> SSETWRFDDGASLSYDWAAHRYRVELPSGTVEVRVGASEVRVSDGAVSLKAPKISLEGPVEIAGTL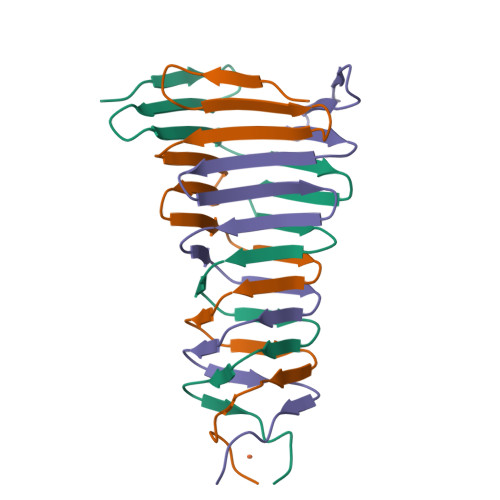TVSGDILGGGSIIDTAGNSNHHTH>MTIDEIIEAIEKLTVSELAELVKKLEDKFGVTAAAPVAVAAAPVAGAAAGAAQEEKTEFDVVLKSFGQNKIQVIKVVREITGLGLKEAKDLVEKAGSPDAVIKSGVSKEEAEEIKKKLEEAGAEVELK[2x];>MTIDEIIEAIE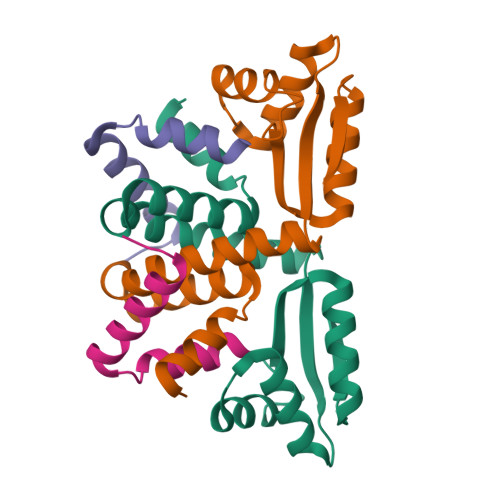KLTVSELAELVKKLEDKFGVT[2x]> MKVKSKPLTLYNVSGDRITADVHFVESFLPAPVVIYSHGFLGFKDWGFIPYVAERFAENGFVFVRFNFSHNGIGENPNKITEFDKLAKNTISKQIEDLTAVIEYVFSDEFGVLNDGQLFLLGHSGGGGISIIKAVEDERVRALALWASISTFRRYSKHQIEELEKNGYIFVRVPDSVIQVKIEKIVYDDFVENSERYDIIKAISKLKIPILIVHGTADAIVPLAEAEKLRNSNPEYTKLVLISGANHLFNVKHPMEHSTDQLDKA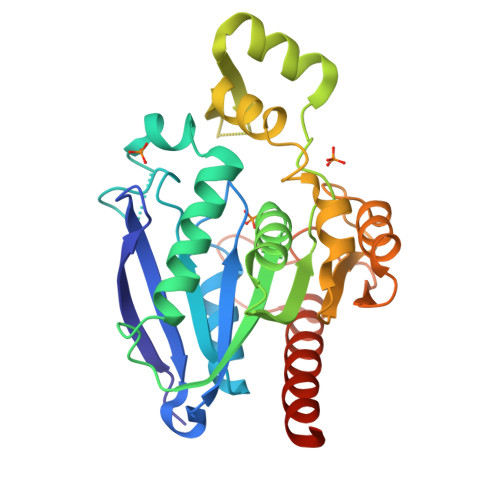IDETVLFFKKIIENKKADLEHHHHHH>[10x]MPGSIPLIGERFPEMEVTTDHGVIKLPDHYVSQGKWFVLFSHPADFTPVCTTEFVSFARRYEDFQRLGVDLIGLSVDSVFSHIKWKEWIERHIGVRIPFPIIADPQGTVARRLGLLHAESATHTVRGVFIVDARGVIRTMLYYPMELGRLVDEILRIVKALKLGDSLKRAVPADWPNNEIIGEGLI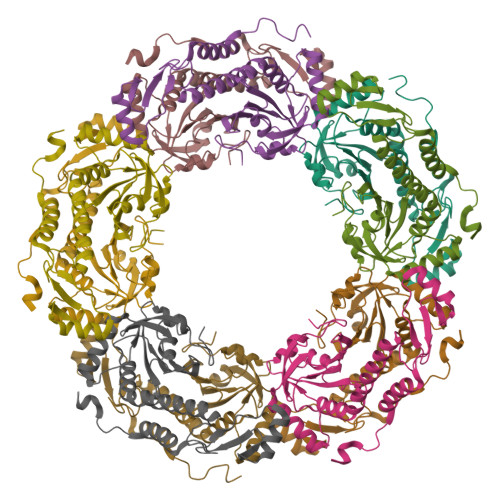VPPPTTEDQARARMESGQYRSLDWWFCWDTPASRDDVEEARRYLRRAAEKPAKLLYEEARTHLH>MNISD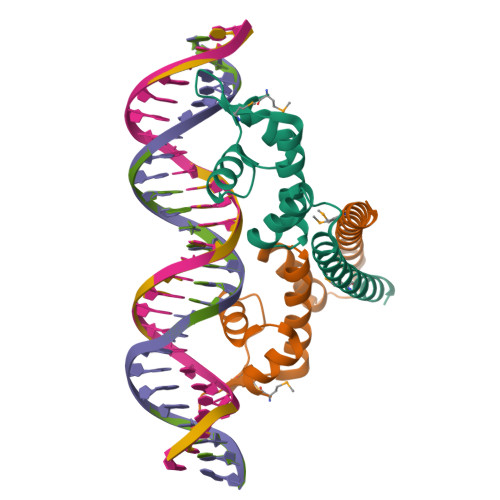VAKITGLTSKAIRFYEEKGLVTPPMRSENGYRTYTQQHLNELTLLRQARQVGFNLEESGELVNLFNDPQRHSADVKRRTLEKVAEIERHIEELQSMRDQLLALANASPGDDSADSPIIENLSG[2x]> MKLLSTYRLQPM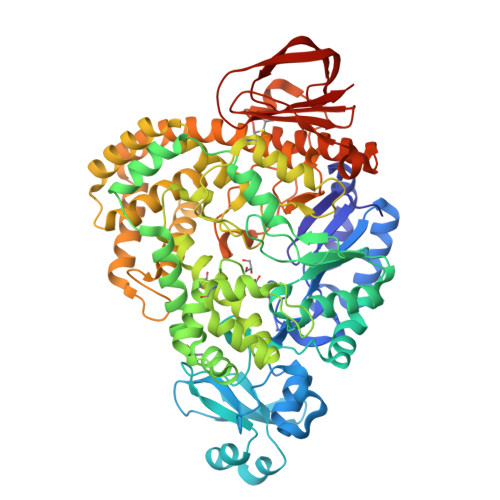KFSEIRNRLDYFVELGVTHLYLSPVLKARPGSTHGYDVVDYNTINDELGGEEEYIRLIDEAKSKGLGIIQDIVPNHMAVHHTNWRLMDVLKKGRHSRYYNYFDFYEEEEKIRIPILGDRNFKITYVNDEPYLDYYGNLFPINDEGRNYLNDIEKLLKVQYYELVDWRDYPSYRRFFAVNELIAVRQELEWVFEDSHSKILSFEVDGYRIDHIDGLFKPEEYLRRLKNKIGNKHIFVEKILSIGEKLRWDFIDGTTGYDFLNYSNLLFTDNEDKMTEIYKNILDIDLDELVKETKKKIIDTLFKHDIERISMMLGVNYEEIKEFLSCLKVYRTYITENDFRDEEIIRNCSQKVYESMKKNVTAFMKLQQYMPAVFAKAYEDTVLFIYNRLISLNEVGSDLHYYSISCDKFHEFNLKRVGTLSFNATSTHDTKFSEDVRMRISAISEIPDEWAKKVNEWHNILNPNIDKNDEYRLYQTIVGSFDGFNNEYKERLKAHMIKALREAKVHTDWVNVNTEYEKKMTYLIDKMFNNEKFMESFLEFESKIDKMGKVKSLSLVALKITSPGVADFYQGLENFRYLLTDPDNRRPVVFSELPKRYEEGLFNNGRIKAYVTKVLLNLRKSMKDFFINSEYKPLKLQKGLCGFMRGDKVLVIVKTLNRDYDIEIDGEYTDVITDETVRGRVKVDKLPLILVK>[3x]GSHMDHLPMPKFGPLAGLRVVFSGIEIAGPFAGQMFAEWGAEVIWIENVAWADTIRVQPNYPQLSRRNLHALSLNIFKDEGREAFLKLMETTDIFIEASKGPAFARRGITDEVLWQHNPKLVIAHLSGFG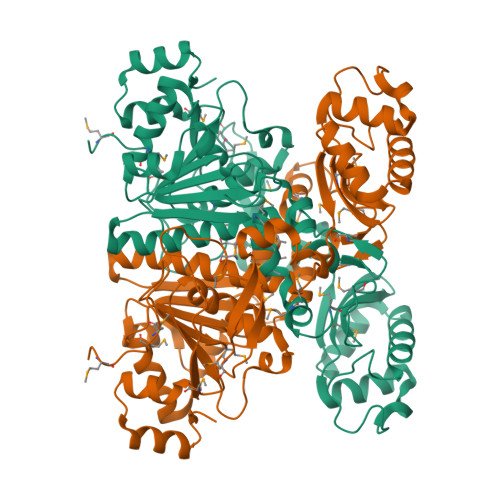QYGTEEYTNLPAYNTIAQAFSGYLIQNGDVDQPMPAFPYTADYFSGLTATTAALAALHKVRETGKGESIDIAMYEVMLRMGQYFMMDYFNGGEMCPRMSKGKDPYYAGCGLYKCADGYIVMELVGITQIEECFKDIGLAHLLGTPEIPEGTQLIHRIECPYGPLVEEKLDAWLATHTIAEVKERFAELNIACAKVLTVPELESNPQYVARESITQWQTMDGRTCKGPNIMPKFKNNPGQIWRGMPSHGMDTAAILKNIGYSENDIQELVSKGLAKVED>[2x]XPVGARGPAGPQGPRGDKGETGEQGDRGIKG;>[4x]XA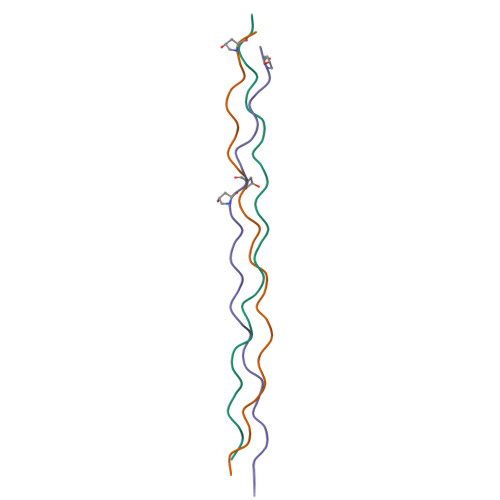VGPRGPSGPQGIRGDKGEPGEKGPRGLPG>KKVISQTVRVDIEKLDNLMDLMGELVIARSRILETLK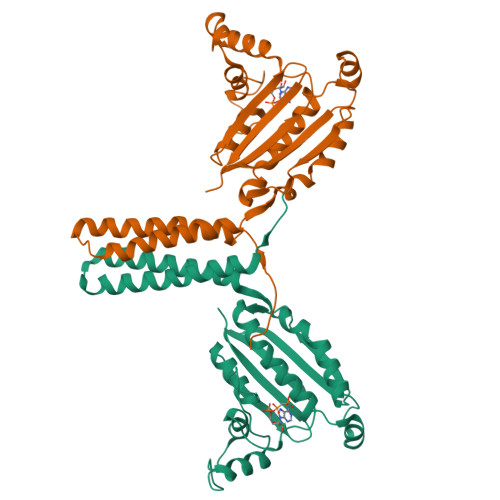KYNIKELDESLSHLSRITLDLQNVVMKIRMVPISFVFNRFPRMVRDLAKKMNKEVNFIMRGEDTELDRTFVEEIGEPLLHLLRNAIDHGIEPKEERIAKGKPPIGTLILSARHEGNNVVIEVEDDGRGIDKEKIIRKAIEKGLIDESKAATLSDQEILNFLFVPGFSTKEKVSEVSGRGVGMDVVKNVVESLNGSISIESEKDKGTKVTIRLPLT[2x]> SMSVPQTKAELLLAIDKNFSKLISYLNTIPPEITSDKSMDGHAKGTEMSVRDLVSYLLGWNALVVKWIASDAKGLPVDFPET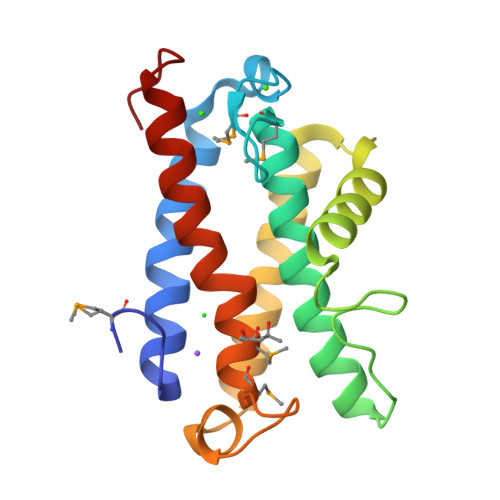GYKWNQLGLLAQKFYSDYSELSYELLVAELQTVKNEIVNLINDRTDDILYGRPWYTKWTMGRMISFNTSSPYANANGRLRKWAKNNNISLK>[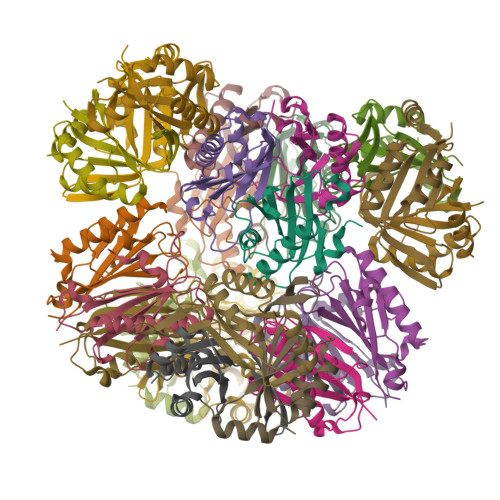12x]GGEEVVLITVPSALVAVKIAHALVEERLAACVNIVPGLTSIYREEGSVVSDHELLLLVKTTTDAFPKLKERVKELHPYEVPEIVALPIAEGNREYLDWLRENTGLE;>[12x]GSVRGIRGAITVEEDTPAAILAATIELLLKMLEANGIQSYEELAAVIFTVTEDLTSAFPAEAARLIGMHRVPLLSAREVPVPGSLPRVIRVLALWNTDTPQDRVRHVYLNEAVRLRPDLESAQLE3-[2-(6-amino-4-methylpyridin-2-yl)ethyl]-5-[3-(methylamino)propyl]benzonitrile 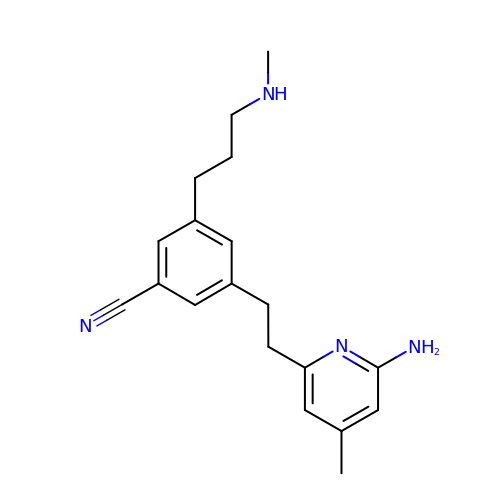| C19 H24 N4 | ZTTVVSIEPMOZBM-UHFFFAOYSA-N> VEKLTADAELQ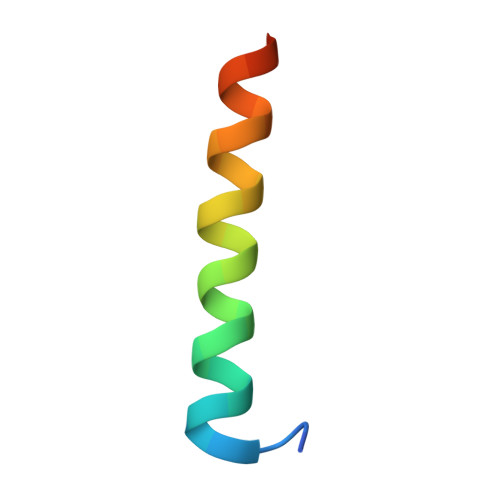RLKNERHEEAELERLKSEY> PAARVEYIAPWWVVWLHSVPHLGLRLQRVDSTFSPGDETYQESLLFLGVLAAIGLGLNLIFLTVYLVCTCCCRRDHTVQTKQQESCCVTWTAVVAGLLCCAAVGVGFYGNSETNDGMHQLIYSLDNANHTFSGMDELVSANTQRMKVDLEQHLARLSEIIAARGDYIQTLKFMQQMAGNVVSQLSGLPVWREVTTQLTKLSHQTAYVEYYRWLSYLLLFILDLVICLVTCLGLARRSKCLLASMLCCGILTLILSWASLAADAAAAVGTSDFCMAPDIYILNNTGSQINSEVTRYYLHCSQSLISPFQQSLTTFQRSLTTMQIQVGGLLQFAVPLFPTAEKDLLGIQLLLNNSEISLHQLTAMLDCRGLHKDYLDALTGICYDGIEGLLFLGLFSLLAALAFSTLTCAGPRAWKYFINRDRDYDDIDDDDPFNPQARRIAAHNPTRGQLHSFCSYSSGLGSQCSLQPPSQTISNAPVSEYMNQAILFGGNPRYENVPLIGRGSPPPTYSPSMRPTYMSVADEHLRHYEFPSSNSLEVLFQ

Tweety homologs (TTYHs) are conserved transmembrane proteins present in all eukaryotes including three members (TTYH1, TTYH2, and TTYH3) in humans. TTYHs have been reported to form Ca2+- and cell volume-regulated anion channels structurally distinct from any characterized protein family with potential roles in cell adhesion, migration, and developmental signaling. Each protomer consists of five transmembrane helices (TM1–5) and an extracellular domain (ED) which extends 75 Å from the membrane surface between an extracellular N-terminus and intracellular C-terminus. We conclude TTYHs are not pore forming subunits of anion channels and their function may involve Ca2+-dependent changes in quaternary structure, interactions with hydrophobic molecules near the extracellular membrane surface, and/or association with additional protein partners.

To test this, we purified and reconstituted TTYH2 into lipid nanodiscs without Ca2+ and in the presence of EGTA to maintain low free Ca2+ concentrations for structure determination. We also pretreated filter paper used for EM grid blotting with EGTA to sequester the high residual Ca2+ known to be present in this material to prevent Ca2+ transfer to the TTYH2 nanodisc sample. The Ca2+-free TTYH2 cryo-EM data did reveal a change in oligomeric state, but surprisingly we identified two different conformations in approximately equal proportions: the expected monomeric TTYH2 (to 4.0 Å resolution) and an unexpected head-to-head homodimer (a “trans-dimer” to 3.9 Å resolution) in which TTYH2 protomers embedded in separate nanodiscs associate via a buried surface at the distal end of each ED. Protomers within monomeric, trans-dimeric, and cis-dimeric TTYH2 adopt overall very similar conformations (pairwise protomer r.m.s.d. = 1.3–1.5 Å) with conformational changes largely limited to subtle rearrangements of side chains. The pocket and unassigned density is similarly observed in TTYH3 cis-dimers, TTYH2 monomers, and TTYH2 trans-dimers, suggesting it may be a conserved site for binding small molecules or extended and primarily apolar lipid headgroups. In contrast, it is exposed in TTYH2 cis-dimers and monomers with ~250 Å2 of solvent accessible area presented to solution by each RGD. Notably, reported human TTYH1 and TTYH2 structures determined in Ca2+-free conditions are also cis-dimers, while we observe monomers and trans-dimers of mouse TTYH2 prepared in Ca2+-free conditions here. For dissociation of cis-dimers into monomers, these include: (1) the affinity of TTYHs for Ca2+, (2) the related dependence of TTYH oligomeric state changes on [Ca2+]ext, and (3) the range of [Ca2+]ext experienced by TTYH-expressing cells under different conditions.>MELWLVRHGETLWNREGRLLGWTDLPLTAEGEAQARRLKGALPS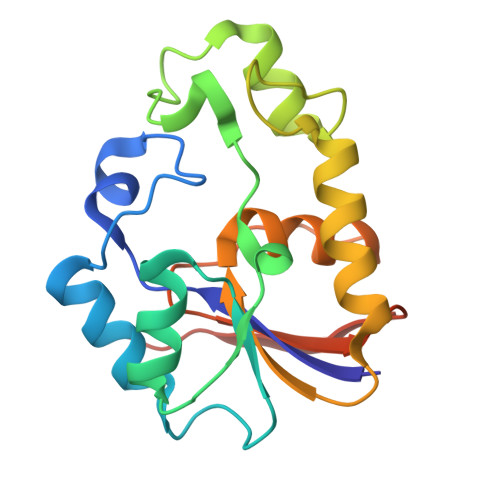LPAFSSDLLRARRTAELAGFSPRLYPELREIHFGALEGALWETLDPRHKEALLRFQGFHPPGGESLSAFQERVFRFLEGLKAPAVLFTHGGVVRAVLRALGEDGLVPPGSAVAVDWPRRVLVRLALDGEEATG[2x]> SPTAEACGYSDRVAQLTVGNSTITTQEAANVIVAYGEWPQYCPDTDATAVDKPTRPDVSVNRFYTLDTKDWSSSSKGWYWKFPDILAETGVFGQNAQFHFLYRSGFCIHVQCNA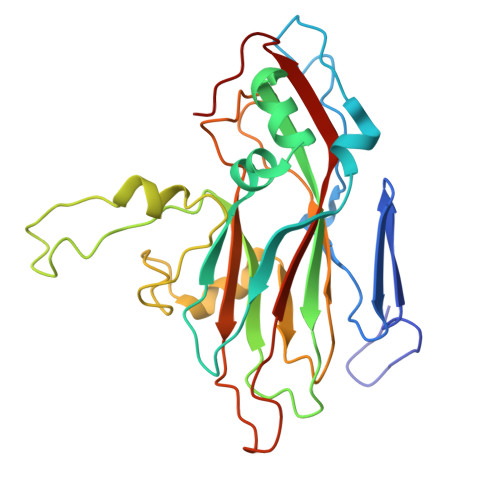SKFHQGALLVAVLPEYVTGTVSGNTGHENTHPPYAATQPGATGFELTNPYILDAGIPLSQLLVCPHQWINLRTNNCATIVVPYINSVPFDSALNHCNFGLVVIPVSPLGFLQGATPTIPITITVAPMNSEFSGLRQAVTQ>[3x]GDEQSEAQFFAPTKESPYEGIPGRLRYNVRIVLVEQDKQGNYIARRDSSTVSKRQLAATVIAAARYYAQEKRAA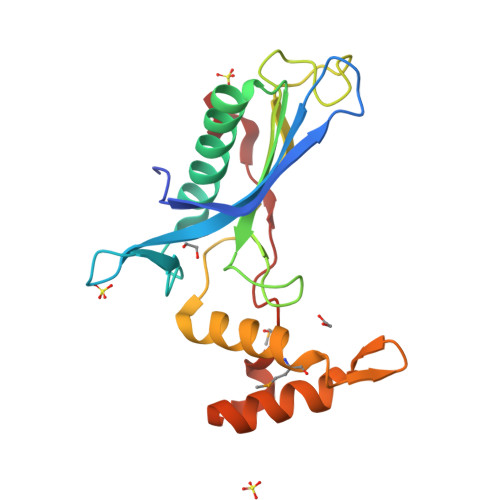VVSITLDSQPGPAFGKTVLATATYAPDGKGVSGSDDWTWNTLQATPRGLTAQELKIQCLWGEMRGKFQVDGSTDERRLKAAIAKKLKIPAEKVMLNPVFPEPFPQEWTR> GTSSMADIGTTNDALDYYLKSKGFNGLFSQIELSFSASNLRDRDVLSKSDPMVVVYQKEKDATLSEVFRSEVVLNSLAPKWIKKFIVAYHFETVQTLVFRVYDVDTKFQNSREEMLKLDEQQFLGEATCALSEIITKSTRTSTLELKRKDGFAPQAQPHHGKLIIHAEESLASKISTEIVFRCSNLESKDLFSKSDPFLVVSKIVEHGT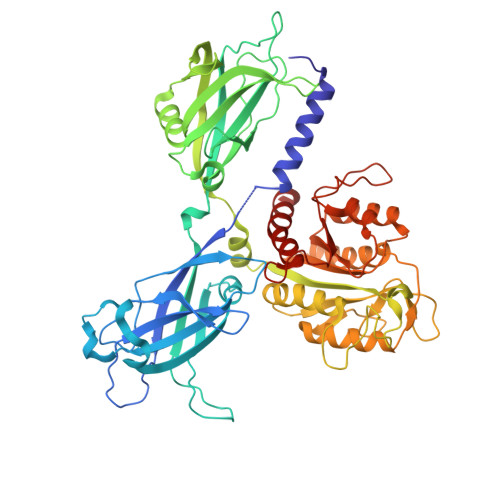PIPVSKTEVRKNDLNPIWKPVFLSVQQVGSKDSPVIIECSDFNSNGKHSLIGKVQKSLSDLEKLHLAGQGINFSLPTGAGQNKVLKSQLFVDKFTETVHHTFLEYLASGFELNFMVAIDFTASNGNPRLPDSLHYIDPSGRLNAYQRAIMDVGEVLQFYDSDKRFPAWGFGARPIDAPVSHCFNLNGSSSYSEVDGIQGIMTSYTSALFNVSLAGPTLFGPVINAAAMIASASLAQGSRKYYVLLIITDGVITDLQETKDALVSASDLPLSILIVGVGGADFKEMEILDADKGERLESSSGRLASRDIVQFVALRDVQYGEISVVQALLAELPSQFLTYMRIRN(2,4-dihydroxyphenyl)(4-hydroxyphenyl)methanone 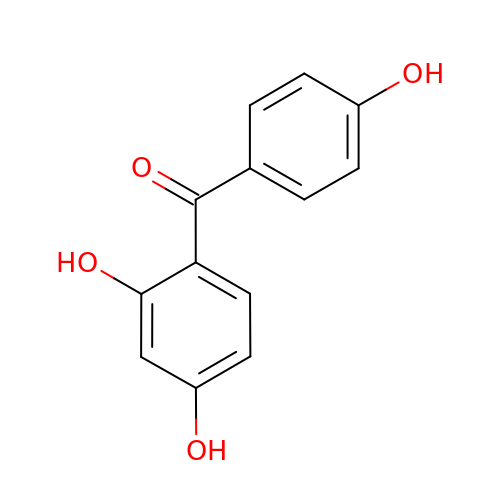| C13 H10 O4 | OKJFKPFBSPZTAH-UHFFFAOYSA-N> MVTENPQRLTVLRLATNKGPLAQIWLASNMSNIPRGSVIQTHIAESAKEIAKASGSDDESGDNEYITLRTSGELLQGIVRVYSKQATFL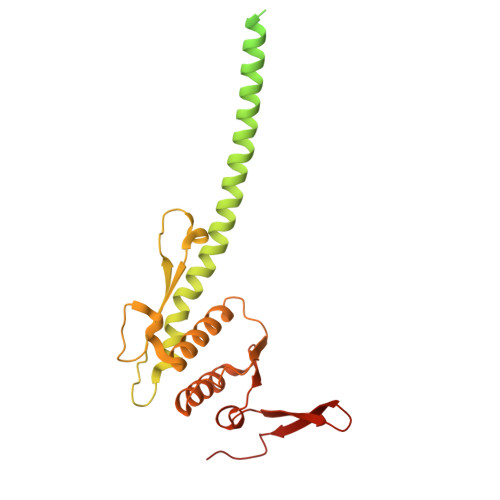LTDIKDTLTKISMLFKTSQKMTSTVNRLNTVTRVHQLMLEDAVTEREVLVTPGLEFLDDTTIPVGLMAQENPNLRAMDRLDHVRKQLEQTEQEFEASKAKLRQARESFQAVKQKRLELFNKAFTHIQEQITHVYKELTRSEAYPLGGQAYLDIEEDTDTPFLSGVKYHAMPPCKRFRDMEHLSGGEKTMAALALLFAIHSYQPSPFFVLDEVDCALDNANVEKIKKYIREHAGPGMQFIVISLKPALFQASESLIGVYRDQEANTSRTLTLDLRKYRHHHHHH>[6x]GPGGEDVIDSLQLNELLNAGEYKIGELTFQSIRSSQELQKKNTIVNLFGIVKDFTPSRQSLHGTKDWVTTVYLWDPTCDTSSIGLQIHLFSKQGNDLPVIKQVGQPLLLHQITLR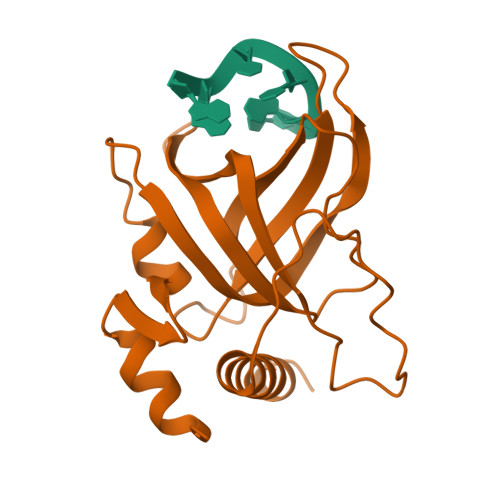SYRDRTQGLSKDQFRYALWPDFSSNSKDTLCPQPMPRLMKTGDKEEQFALLLNKIWDEQTNKHKNGELLSTS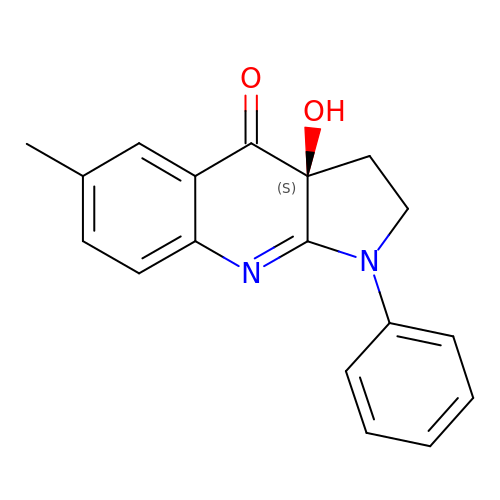(-)-1-PHENYL-1,2,3,4-TETRAHYDRO-4-HYDROXYPYRROLO[2,3-B]-7-METHYLQUINOLIN-4-ONE | C18 H16 N2 O2 | LZAXPYOBKSJSEX-GOSISDBHSA-N> STKYPIVLVHGLAGFNEIVGFPYFYGIADALRQDGHQVFTASLSAFNSNEVRGKQLWQFVQTLLQETQAKKVNFIGHSQGPLACRYVAANYPDSVASVTSINGVNHGSEIADLYRRVMRKDSIPEYIVGKVLNAFGTIISTFSGHRGDPQDAIAALESLTTEQV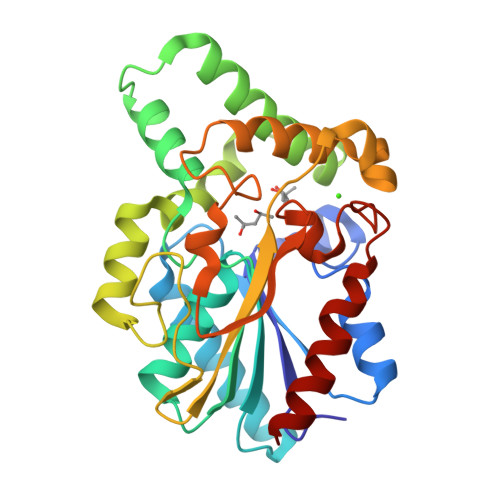TEFNNKYPQALPKTPGGEGDEIVNGVHYYCFGSYIQGLIAGEKGNLLDPTHAAMRVLNTFFTEKQNDGLVGRSSMRLGKLIKDDYAQDHIDMVNQVAGLVGYNEDIVAIYTQHAKYLASKQL>[2x]SNAMARVALLADRLRVEERLLIEAFAARGHEAVLVQPAKLALSPAAPSAGDFVAALDRGEATAERAVLAALLASGGTPVVNRAATARLLADRMALLRHLILADIPVPETRVCFGEEAIFAAIAEIGYPVVLKSLTVDPGFPVALVEDQDAAEAIVEHRIMLGGERAVLVQQFIPARAGQSVRLVVAGRSLAGIEQRTHGGWRPGRDAT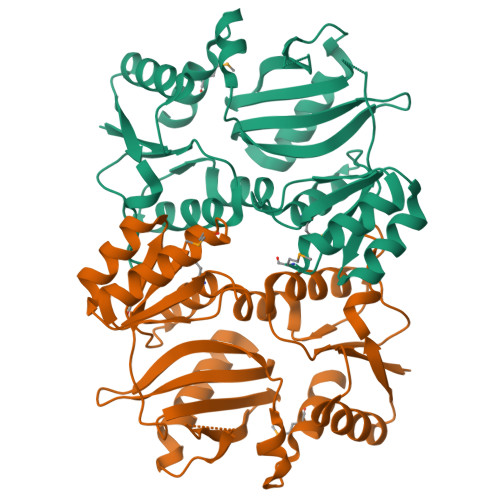YEAYTGDPAPLTALAERIIERLGTGTYAVEVVETGDGPVVVGVANLVDFRSLSGRGVDVAGMIADFVLG>[4x]MANSCDFRVFLQEFGTTVHLSLPGSVSEKERLLLKLLMQGMSVTEISQYRNRSAKTISHQKKQL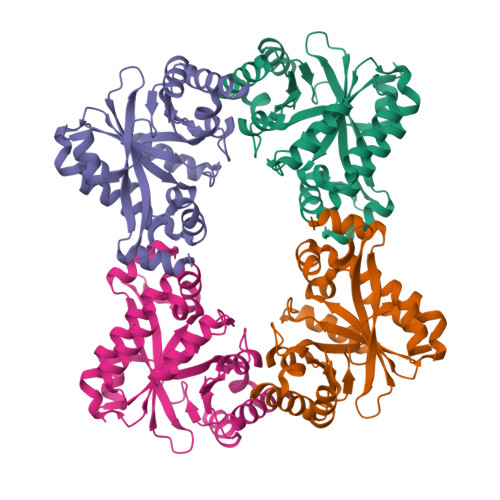FEKLGIQSDITFWRDIFFQYNPEIISATGSNSHRYINDNHYHHIVTPEAISLALENHEFKPWIQPVFCAQTGVLTGCEVLVRWEHPQTGIIPPDQFIPLAESSGLIVIMTRQLMKQTADILMPVKHLLPDNFHIGINVSAGCFLAAGFEKECLNLVNKLGNDKIKLVLELTERNPIPVTPEARAIFDSLHQHNITFALDDFGTGYATYRYLQAFPVDFIKIDKSFVQMASVDEISGHIVDNIVELARKPGLSIVAEGVETQEQADLMIGKGVHFLQGYLYSPPVPGNKFISEWVMKAGGHHHHHH Ubiquinone-8 | C49 H74 O4 | 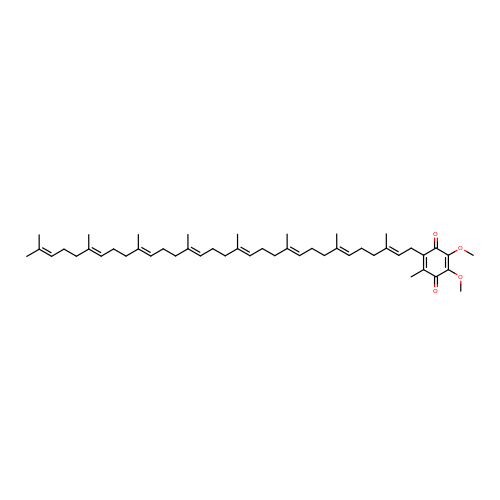ICFIZJQGJAJRSU-SGHXUWJISA-N> 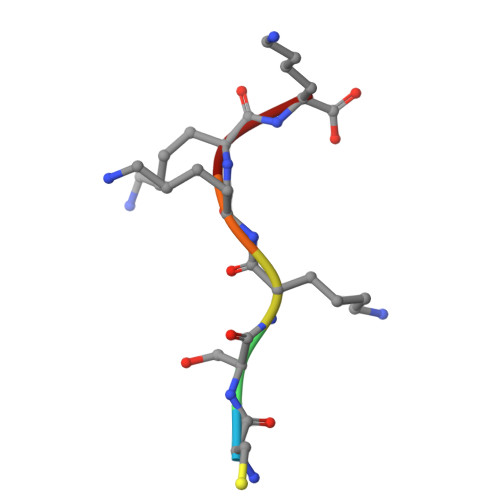CSKKKK>ETGIGTLIIFIAMVLVAAVAATVLINTAGSLQQRATSTGSQTTNQVSTGLIVQSIYGMDNNRSNPESGSLNWTAIYVTLNTGSSPVDLSNVSLSLEYQGQLASLKYTPATTNASFAVDTNGTSNVFSVLNAGVGYKNSTATFKNVELKNVTKSTNFAIVVIRDPSNSLTSSHPVLTTGSEVVILVNTSAVFGGMKQGQAVTGQINPSVGSPGIIQFTTPSAFTETVMELQ[33x]

Archaeal Type IV pilins and archaellins, which form the subunits of pili and archaella, respectively, are expressed as preproteins with a signal peptide. The pilins/archaellins are then assembled into a filament, wherein the hydrophobic alpha helical N-termini are helically stacked in the core of the filament, and the hydrophilic β-strand-rich heads are oriented towards the filament's periphery. Through single particle cryo-electron microscopy (cryoEM) and helical reconstruction, we solved the structures of these filaments at 2.61 and 2.52 Å resolution for C. divulgatum and O. meridianum, respectively. Atomic model building, bioinformatics analysis, and motility experiments suggest that the C. divulgatum fibre is a nonrotary, likely adhesive T4P, whereas the O. meridianum filament is an archaellum.

The ArlB of O. meridianum is largely a typical archaellin, consisting of an N-terminal α-helical tail and a globular head domain. The O. meridianum pre-archaellin ArlB has a length of 254 AA, of which the 26 most N-terminal residues form the leader peptide. The O. meridianum archaellum filament has an unusual, barbed structure distinct from previously investigated archaella, which tend to have a rather smooth surface. The barbs are formed by a unique extended loop that is flanked by two short ⍺-helices and spans from V126 to L153. In the assembled filament, these spikes give the archaellum a barbed surface profile. Oxyplasma meridianum ArlB boasts eight glycans (N62, N72, N91, N113, N121, N138, N150, N187), making it the most heavily glycosylated archaeal filament protein known to date. Nine N-glycosylation sequons are present in total; however, N206 faces inside the β-sheet head and thus is likely inaccessible to posttranslational modification. Only two of the eight glycans are bound to the spike domain, suggesting that it has not evolved to serve as a dedicated glycosylation sub-domain, as seen in the archaellum of S. acidocaldarius. In contrast, a typical hinge region for archaella consists of two residues, and the archaellum of O. meridianum follows this general trend. We observed that O. meridianum is capable of directional swimming motion, thus confirming that the archaella of this organism are indeed functional.>MAKLNMNNEIKKVEQRLEKAIKSKDSVLEQASLHLLSSGGKRVRPAFVILSSQFGKDEQTSEQTYQVAVALELIHMATLVHDDVIDKSDKRRGKLTISKKWDQTTAILTGNFLLALGLEHLMAVKDNRVHQLISESIVDVCRGELFQFQDQFNSQQTIINYLRRINRKTALLIQISTEVGAITSQSDKETVRKLKMIGHYIGMSFQIIDDVLDFTSTEKKLGKPVGSDLLNGHITLPILLEMRKNPDFKLKIEQLRRDSERKEFEECIQIIRKSDSIDEAK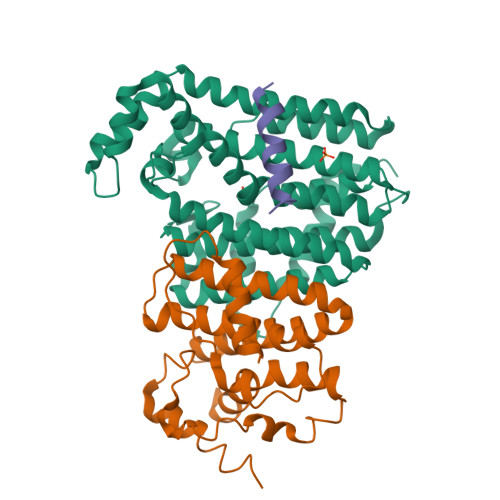AVSSKYLSKALNLISELPDGHPKSLLLSLTKKMGSRNT[2x];>METTVSKLERQIEERLKGVSEYESININHRLGKLLDSYDIPDVAKVACLTIDTSMRHLDDITYNHLSKHSILIGDLISAHFYTLLAEINDLSFQNEISKAIVEINELKSSLHHQALNDYEISQAIVKIETLFPYITLSHFGINIDESEIYNYLFEDMSDYYPSYFKKYNQSEVKHYLHDIQKSYLKSRGN[2x];>[2x]KHYLHDIQKSYLKSRGN>GMSQFQEVRPVAQALYPTHPSTKDALEEA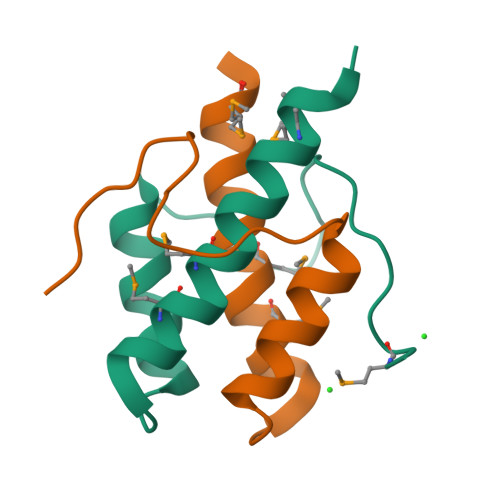RLLFPGGTHHDFMRALMGYHNTLVKVMEEQCGS[4x]2-(2-methoxyethyl)-1,2,3,4-tetrahydroisoquinolin-8-amine 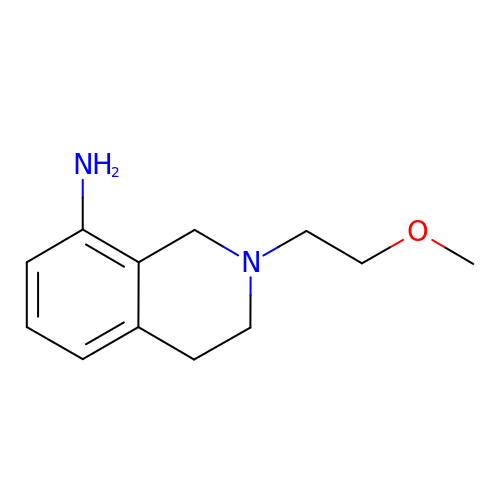| C12 H18 N2 O | IJXQCLYAKMPTMJ-UHFFFAOYSA-N> NSVSVDLPGSMKVLVSKSSNADGKYDLIATVDALELSGTSDKNNGSGVLEGVKADASKVKLTISDDLGQTTLEVFKSDGSTLVSKKVTSKDKSVTFEKFNEKGEVSEKIITRADGTRLEYTGIKSDGSGKAKEVLKGYVLEGTLTAEKTTLVVKEGTVTLSKNISKSGAVSVELNDTDSSAATKKTAAWNSGTSTLTITVNSKKTKDLVFTSS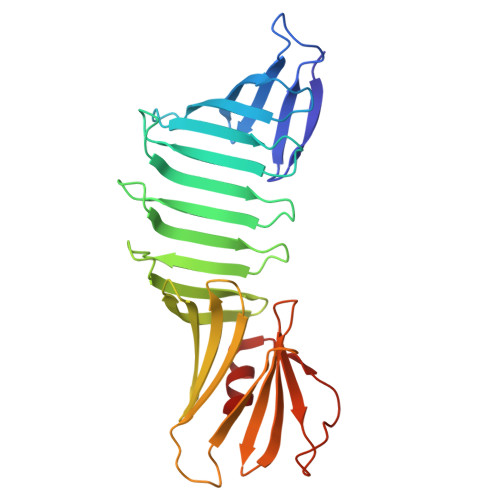NTITVQQYDSNGTSLEGSAVEITKLDEIKNALK> MAPKAKIVLVGSGMIGGVMATLIVQKNLGDVVLFDIVKNMPHGKALDTSHTNVMAYSNCKVSGSNTYDDLAGSDVVIVTAGFTKAPGKSDKEWNRDDLLPLNNKIMIEIGGHIKKNCPNAFIIVVTNPVDVMVQLLHQHSGVPKNKIIGLGGVLDTSRLKYYISQKLNVCPRDVNAHIVGAHGNKMVLLKRYITVGGIPLQEFINNKLISDAELEAIF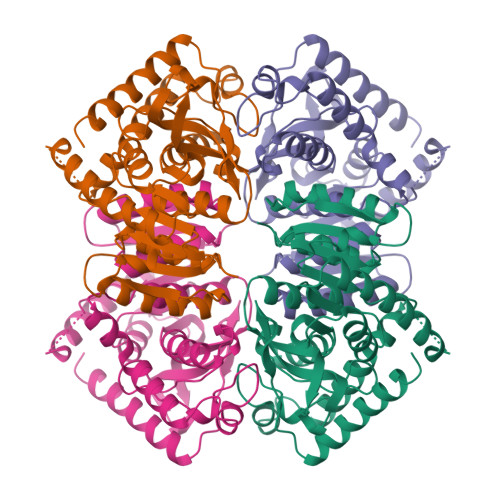DRTVNTALEIVNLHASPYVAPAAAIIEMAESYLKDLKKVLICSTLLEGQYGHSDIFGGTPVVLGANGVEQVIELQLNSEEKAKFDEAIAETKRMKALA>[2x]MRSRRVD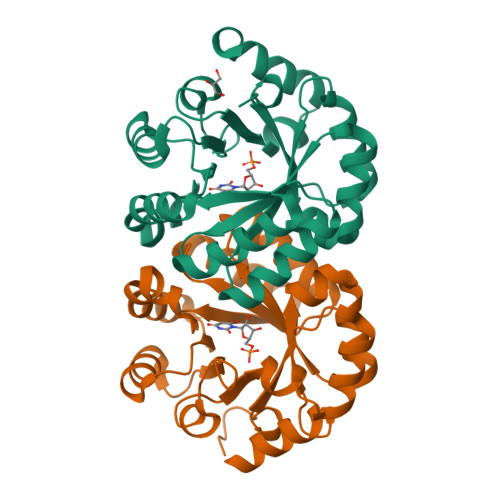VMDVMNRLILAMDLMNRDDALRVTGEVREYIDTVKIGYPLVLSEGMDIIAEFRKRFGCRIIADFKVADIPETNEKICRATFKAGADAIIVHGFPGADSVRACLNVAEEMGREVFLLTEMSHPGAEMFIQGAADEIARMGVDLGVKNYVGPSARPERLSRLREIIGQDSFLISPGVGAQGGDPGETLRFADAIIVGRSIYLADNPAAAAAGIIESIKDLLNP>[3x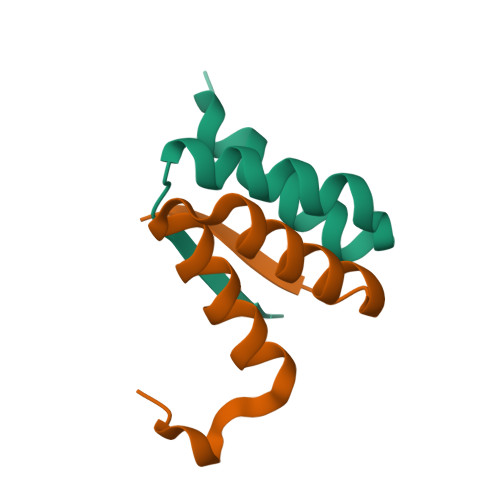]YRSPGNLTEREELAGSLARAIAGGDEKGAAQVAAVLAQHRVALSVQLQ>MDERIQALRKEVDRVNREILRLLSERGRLVQEIGRLQTELGLPHYDPKREEEMLAYLTAENPGPFPDETIRKLFKE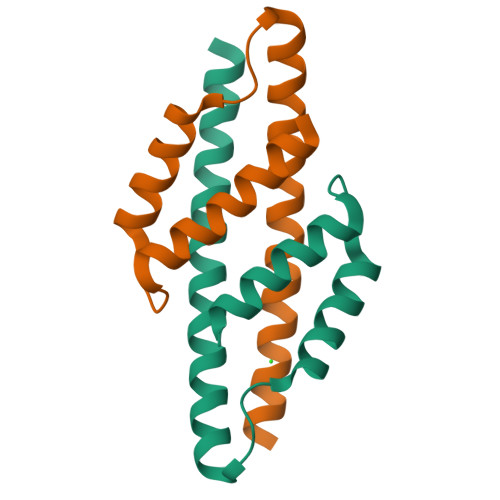IFKASLDLEERQDQ[2x]2-AMINO-4-METHYLTHIAZOLE 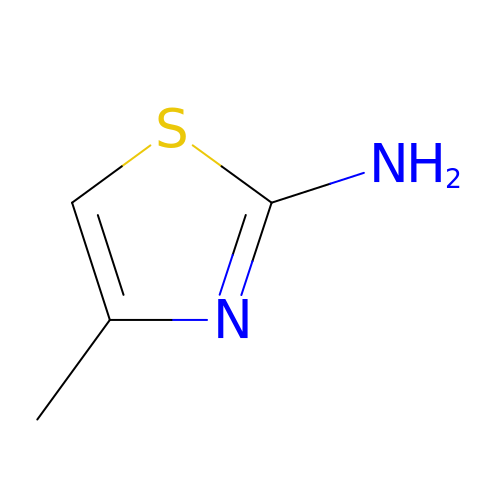| C4 H6 N2 S | OUQMXTJYCAJLGO-UHFFFAOYSA-N2-methyl-5-phenyl-pyrazol-3-amine | C10 H11 N3 | 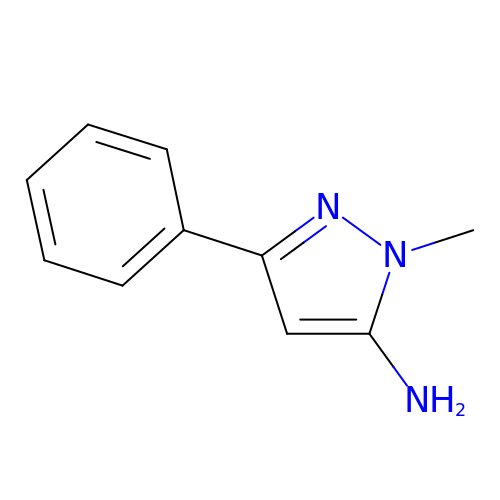KCYRMURRLLYLPU-UHFFFAOYSA-N> MHHHHHHSSGRENLYFQGCQVIAMYDYAANNEDELSFSKGQLINVMNKDDPDWWQGEINGVTGLFPSNYVKMTTDSDPSQQWCADLQTLDTMQPIERKRQGYIHELIQTEERYMADLQLVVEVFQKRMAESGFLTEGEMALIFVNWKELIMSNTKLLKALRVRKKTGGEKMPVQMIGDILAAELSHMQAYIRFCSCQLNGAALLQQKTDEDTDFKEFLKKLASDPRCKGMPLSSFLLKPMQ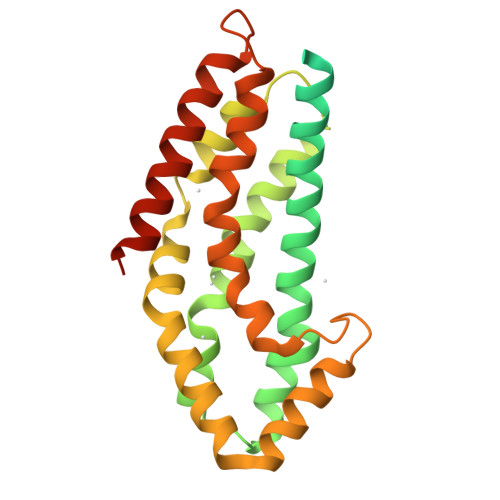RITRYPLLIRSILENTPESHADHSSLKLALERAEELCSQVNEGVREKENSDRLE4-(8-fluoranyl-6-oxidanylidene-1,3,4,5-tetrahydrobenzo[c][1,6]naphthyridin-2-yl)butanoic acid | C16 H17 F N2 O3 | 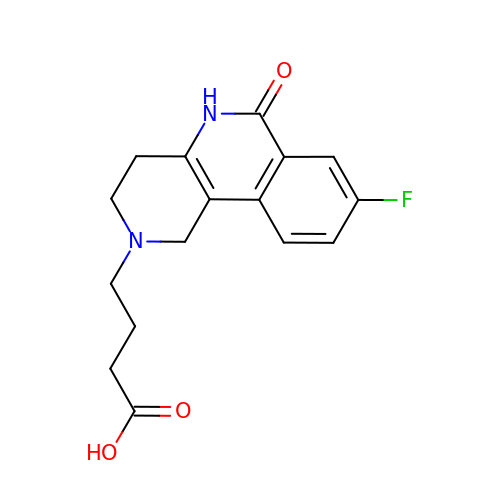HXURHTYUPWDBOT-UHFFFAOYSA-N For rotaviruses (RVs), which are the major causative agents of life-threatening gastroenteritis in children under the age of 5 years and result in 453,000 deaths worldwide annually, recognition of specific cellular glycans for initial cell attachment is mediated by the distally located VP8* domain of the spike protein VP4. Although structurally conserved with a galectin-like fold, sequence-wise VP8* is the least conserved among RV structural proteins contributing to a phylogeny consisting of 37 [P] genotypes9. Our crystallographic analyses provide the structural basis to explain the unique glycan specificity exhibited by a neonate-specific bovine-human reassortant RV strain and its parental bovine strain, each belonging to the P genotype. We have shown that P VP8* exhibits a novel glycan-binding site that adapts to a differential recognition of precursor glycans, which are the core elements of HBGA and human/bovine milk glycans.

The residues interacting with the type II glycan in the P HRV VP8* are conserved in the BRV VP8*, indicating that the bovine VP8* can also bind glycans with the β1,4 motif using the same binding site. To test our hypothesis that both human and bovine P VP8*s use the same binding site to interact with type II glycan, we co-crystallized bovine P VP8* with LNnT. The crystals, with four molecules in the asymmetric unit, diffracted to 1.46 Å. The crystal structure shows that the Galβ1,4-GlcNAc moieties of LNnT at the non-reducing end interact at the same binding site as in the human P VP8* with similar hydrophobic interactions involving the conserved N155, Y156, W178, G179 and D185 and hydrogen bond interactions involving the conserved R154 and R187. The electron density for the Glc moiety at the reducing end, however, is not well defined in any of the four molecules in the asymmetric unit because of the lack of engagement by the protein and was not modelled in the final structure. Similar to P HRV VP8*, bovine VP8* also undergoes conformational changes upon binding to LNnT including reorientation of the side chains of R154 and R187. In the ligand-bound bovine P VP8* structure, in all the four molecules of the asymmetric unit, the conformation of the J-K loop remains the same as in the apo structure, despite the space group difference, indicating that the different conformation of the J-K loop from that observed in the human P VP8* is mainly due to the sequence variations and not the ligand binding or crystal contacts. Consistent with the structural observation, co-crystallization of P BRV B223 VP8* with LNT using similar concentrations as the LNnT did not show any density for the bound LNT, indicating that LNT cannot bind to B223 VP8*.

>[4x]GSLDGPYAPDSSNLPSNCWYLVNPSNDGVVFSVTDNSTFWMFTYLVLPNTAQTNVTVNVMNETVNISIDNSGSTYRFVDYIKTSSTQAYGSRNYLNTAHRLQAYRRDGDGNISNYWGADTQGDLRVGTYSNPVPNAVINLNADFYVIPDSQQETCTEYIRGGL> MGGGFAGREVSEDVAKQVARSFLNLKGNEQIHIVKSGKDADYEVYSLTITDPKTNQETYMDITQKGGYPLWVLEDRDIKKQNISLNDAMNKATKFLKDHRFESLVMAESAQYDNMGVFTFVEQTESGVRIYPDSVKMKMSLEDGSVIGFSAKDFLLKHRTRDIPKPKISKEQAKTKLNSNVKVMEERLA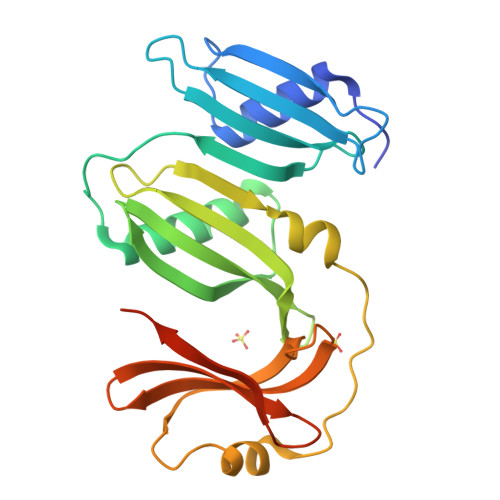IITNDLNEEVLCYEFLGTIKNDTYRIFINADTGFEEKVEKLQNSEPLYNEVENLYFQ> GPVEDAITAAIGRVADTVGTGPTNSEAIPALTAAETGHTSQVVPGDTMQTRHVKNYHSRSESTIENFLCRSACVYFTEYENSGAKRYAEWVLTPRQAAQLRRKL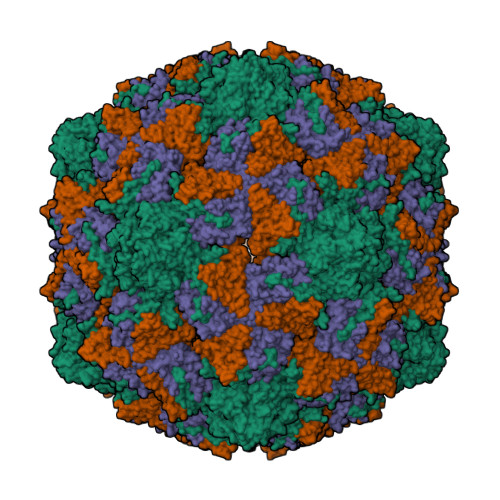EFFTYVRFDLELTFVITSTQQPSTTQNQDAQILTHQIMYVPPGGPVPDKVDSYVWQTSTNPSVFWTEGNAPPRMSIPFLSIGNAYSNFYDGWSEFSRNGVYGINTLNNMGTLYARHVNAGSTGPIKSTIRIYFKPKHVKAWIPRPPRLCQYEKAKNVNFQPSGVTTTRQSITTMTNTGAF;> SPTVEECGYSDRARSITLGNSTITTQECANVVVGYGVWPDYLKDSEATAEDQPTQPDVATCRFYTLDSVQWQKTSPGWWWKLPDALSNLGLFGQNMQYHYLGRTGYTVHVQCNASKFHQGCLLVVCVPEAEMGCATLDNTPSSAELLGGDSAKEFADKPVASGSNKLVQRVVYNAGMGVGVGNLTIFPHQWINLRTNNSATIVMPYTNSVPMDNMFRHNNVTLMVIPFVPLDYCPGSTTYVPITVTIAPMCAEYNGLRLAGHQ;> GLPTMNTPGSCQFLTSDDFQSPSAMPQYDVTPEMRIPGEVKNLMEIAEVDSVVPVQNVGEKVNSMEAYQIPVRSNEGSGTQVFGFPLQPGYSSVFSRTLLGEILNYYTHWSGSIKLTFMFCGSAMATGKFLLAYSPPGAGAPTKRVDAMLGTHVVWDVGLQSSCVLCIPWISQTHYRYVTSDEYTAGGFITCWYQTNIVVPADAQSSCYIMCFVSACNDFSVRLLKDTPFISQQNFFQ2'-O-(sulfidophosphinato)adenosine 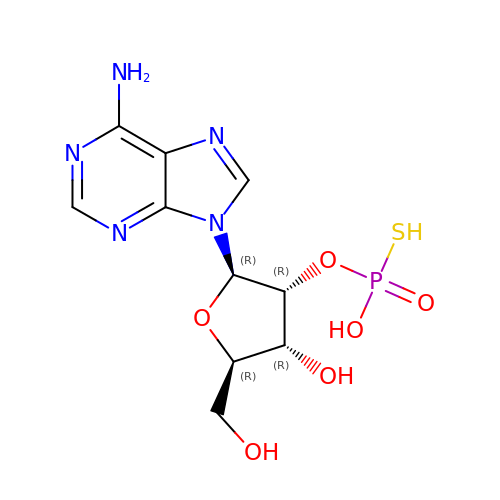| C10 H14 N5 O6 P S | KWODASVFOLWUKA-KQYNXXCUSA-L> SSQIRQNYSTEVEAAVNRLVNLYLRASYTYLSLGFYFDRDDVALEGVCHFFRFLAFFKAFGAFRLLKMQNQRGGRALFQDLQKPSQDEWGTTLDAMKAAIVLEKSLNQALLDLHALGSAQADPHLCDFLESHFLDEEVKLIKKMGDHLTNIQRLVGSQAGLGEYLFERLTLKHD

As a scaffold for aromatic cluster design, we chose ferritin as a protein cage platform with a 12 nm outer diameter and an 8 nm inner cavity, composed of 24 subunits. To prove this concept through protein engineering, we focused on a two‐fold symmetric inter‐subunit interface of a recombinant horse spleen apo‐L ferritin (Fr) as a target region for mutagenesis. Herein, we present the construction of an aromatic cluster with an artificial molecular binding pocket at the two‐fold symmetric interface of ferritin and explore its ligand‐binding characteristics. We developed a system that uses ligand binding as a driving force to induce and propagate changes in the orientation of multiple aromatic side chains.

To modulate the shape of the central pocket, we prepared Fr‐F5/59A (Fr‐E53F/E56F/E57F/R59A/E60F/E63F) and Fr‐F5/59L (Fr‐E53F/E56F/E57F/R59L/E60F/E63F) in which residue 59 was replaced with Ala or Leu (lower). In the case of Fr‐F5/59A, the replacement of Phe59 with alanine (Ala) results in an expanded pocket size. Conversely, in Fr‐F5/59L, the introduction of leucine (Leu) imposes steric hindrance, effectively obstructing the pocket's entrance. These variances in pocket morphology among the variants are anticipated to impact ligand binding affinity and specificity. Replacing Phe59 with Ala or Leu significantly reduced the incorporation amount of NR (1.4 molecules for Fr‐F5/59A and 0.4 molecules for Fr‐F5/59L). Although there was sufficient space for NR in the A59 pocket (distance between A59–A59' 7.9 Å), the substitution of F59 with A59 excluded π–π stacking interactions at the site. As a result, NR has poor affinity to bind at this site in Fr‐F5/59A.> MF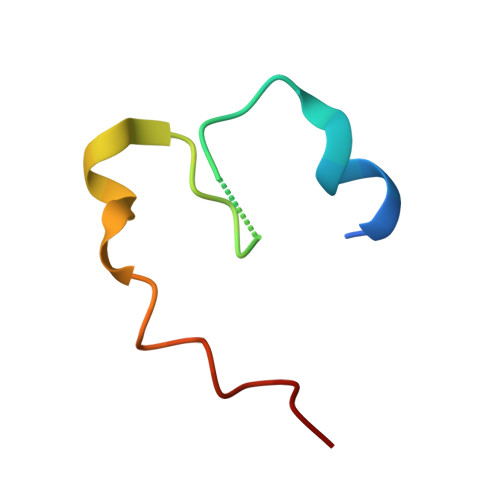DTNATRLPIWGIGCNPWTAEHVDQTLASGNDIC> MPTVDDILEQVGESGWFQKQAFLILCLLSAAFAPICVGIVFLGFTPDHHCQSPGVAELSQRCGWSPAEELNYTVPGLGPAGEAFLGQCRRYEVDWNQSALSCVDPLASLA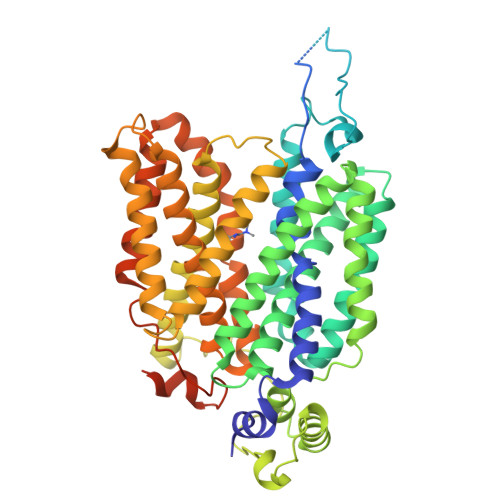TNRSHLPLGPCQDGWVYDTPGSSIVTEFNLVCADSWKLDLFQSCLNAGFLFGSLGVGYFADRFGRKLCLLGTVLVNAVSGVLMAFSPNYMSMLLFRLLQGLVSKGNWMAGYTLITEFVGSGSRRTVAIMYQMAFTVGLVALTGLAYALPHWRWLQLAVSLPTFLFLLYYWCVPESPRWLLSQKRNTEAIKIMDHIAQKNGKLPPADLKMLSLEEDVTEKLSPSFADLFRTPRLRKRTFILMYLWFTDSVLYQGLILHMGATSGNLYLDFLYSALVEIPGAFIALITIDRVGRIYPMAMSNLLAGAACLVMIFISPDLHWLNIIIMCVGRMGITIAIQMICLVNAELYPTFVRNLGVMVCSSLCDIGGIITPFIVFRLREVWQALPLILFAVLGLLAAGVTLLLPETKGVALPETMKDAENLGRKAKPKENTIYLKVQTSEPSGTEDQVDPRLIDGK2-chloro-9-(3-(2,2-difluoroethoxy)-5-(difluoromethoxy)benzyl)-9H-purin-6-amine | C15 H12 Cl F4 N5 O2 | 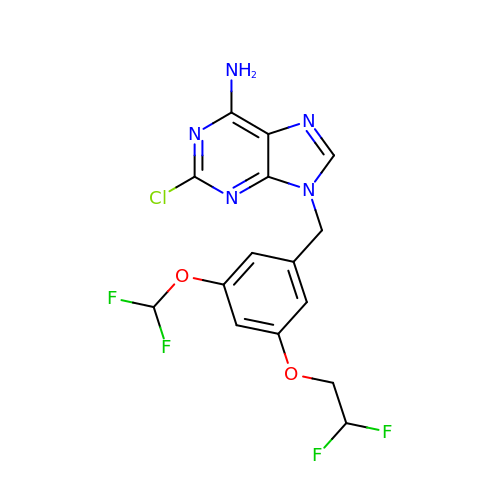DEFIIWXSKZHELC-UHFFFAOYSA-N>[10x]MANLTEKFLRIFARRGKSIILAYDHGIEHGPADFMDNPDSADPEYILRLARDAGFDGVVFQRGIAEKYYDGSVPLILKLNGKTTLYNGEPVSVANCSVEEAVSLGASA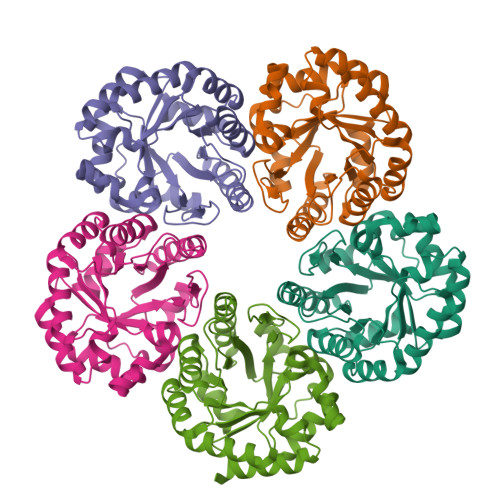VGYTIYPGSGFEWKMFEELARIKRDAVKFDLPLVVWSYPRGGKVVNETAPEIVAYAARIALELGADAMKIKYTGDPKTFSWAVKVAGKVPVLMSGGPKTKTEEDFLKQVEGVLEAGALGIAVGRNVWQRRDALKFARALAELVYGGKKLAEPLNV> MHHHHHHENLYFQGAVPSRSPQASSKSRPLSEQNPPPVWFGEYLSRLRDTYAPELPPPRQFPDPLGGLIRTILSQQNTRRVAQRQWEVLTATYPQWEAALLDGPDGIEATLKSAGGGLSRMKADYIYGILAHLQEHHGGLSLRFLREFPHTPEGHEQARQALAALPGVGHKTVALVLLFDLRRPAMPVDGNMERAAKRLELVPAAWNSHKVERWYAEVMPADWETRFALHISGVRH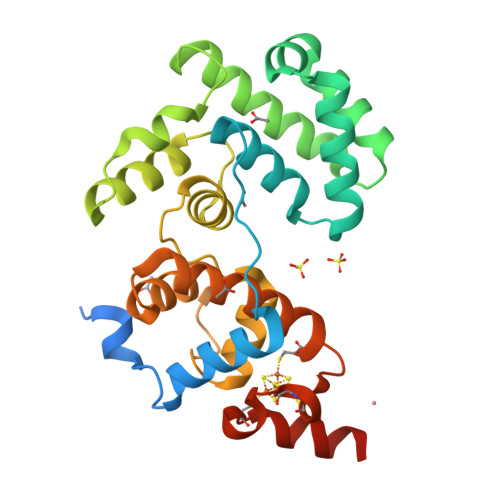GRDTCRSKHPLCPQCPLREFCPSASIFELGEAGEREPSELEW>[8x]MKHHHHHHPMSDKIIHLTDDSFDTDVLKADGAILVDFWAEWCGPCKMIAPILDEIADEYQGKLTVAKLNIDQNPGTAPKYGIRGIPTLLLFKNGEVAATKVGALSKGQLKEFLDANL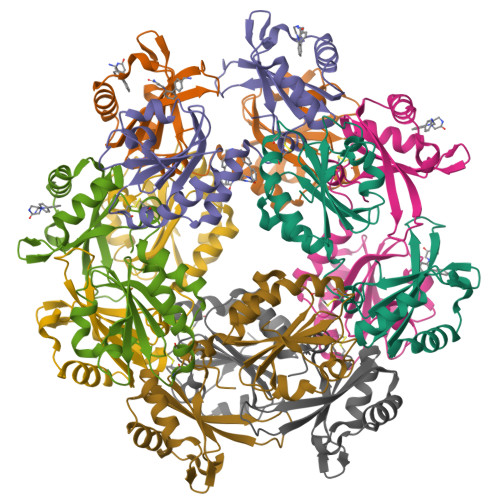AGSAMESTVMVLRNMVDPKDIDDDLEGEVTEECGKFGAVNRVIIYQEKQGEEEDAEIIVKIFVEFSIASETHKAIQALNGRWFAGRKVVAEVYDQERFDNSDLSA> MATTVQLSDQSLRQLETLAIHTAHLIQPHGLVVVLQEPDLTISQISA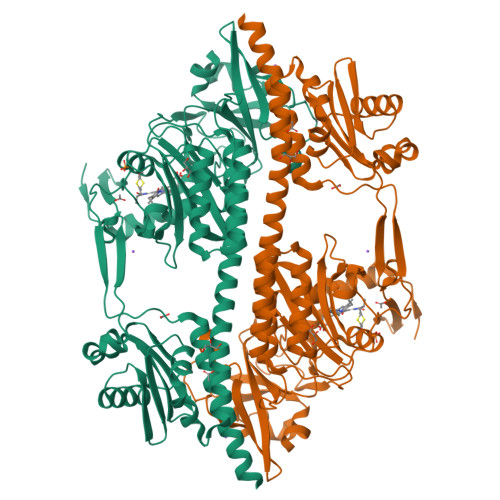NCTGILGRSPEDLLGRTLGEVFDSFQIDPIQSRLTAGQISSLNPSKLWARVMGDDFVIFDGVFHRNSDGLLVCELEPAYTSDNLPFLGFYHMANAALNRLRQQANLRDFYDVIVEEVRRMTGFDRVMLYRFDENNHGDVIAEDKRDDMEPYLGLHYPESDIPQPARRLFIHNPIRVIPDVYGVAVPLTPAVNPSTNRAVDLTESILRSAYHCHLTFLKNMGVGASLTISLIKDGHLWGLIACHHQTPKVIPFELRKACEFFGRVVFSNISAQEDTETFDYRVQLAEHEAVLLDKMTTAADFVEGLTNHPDRLLGLTGSQGAAICFGEKLILVGETPDEKAVQYLLQWLENREVQDVFFTSSLSQIYPDAVNFKSVASGLLAIPIARHNFLLWFRPEVLQTVNWGGDPNHAYEATQEDGKIELHPRQSFDLWKEIVRLQSLPWQSVEIQSALALKKAIVNLILRQAEEHHHHHH> MRGSHHHHHHGSEEASSTGRNFNVEKINGEWHTIILASDKREKIEDNGNFRLFLEQIHVLEKSLVLKFHTVRDEECSELSMVADKTEKAGEYSVTYDGFNTFTIPKTDYDNFLMAHLINEKDGETFQLMGLYGREPDLSSDIKERFAQLCEEHGILRENIIDLSNANRCLQ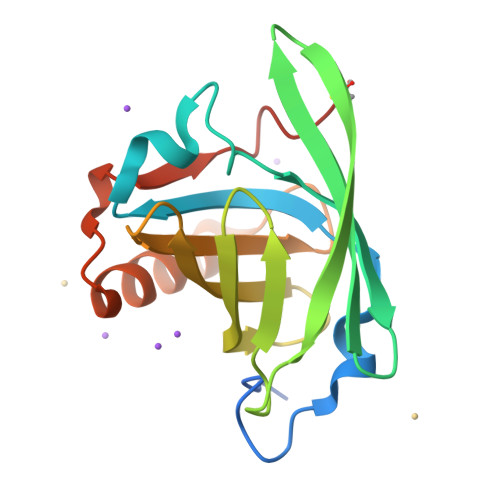ARE>HHHHHHLPEKTIRWCVVSDHEATKCSSFRDNMKKVLPAGGPAVTCVRKMSHPECIRDISANKVDAVTVDGALVAEADLPHHSLKPIMAEYYGSKDDPKTHYYVVAMAKKGTGFQLNQLRGKKSCHTGLGWSAGWYVPLSTLLPSGSRETAAATFFSSSCVPCADGKMFPSLCQLCAGKGTDKCACSSREPYFGSWGALKCLQDGTADVSFVKHLTVFEAMPTKADRDQYELLCMDNTRRPVEEYEQCYLARVPSHVVVARSVDGKEDSIQELLRVAQEHFGKDKSSPFQLFGSPHGEDLLFTDAAHGLLRVPRKIDISLYLGYEFLSAFRNLKRGLEDSQRVKWCAVGQQERTKCDQWSAVSGGALACATEETPEDCIAATMKGEADAMSLDGGFAYVAGHCGLVPVLAENYLSTHSSGRLGSKCVNAPLEGYYVVAVVKKSDVGITWKSLQGKKSCHTAVGTSEGWNVPMGLIYDQTGSCKFDAFFSRSCAPGSDPDSPLCALCVGGNNPAHMCAANNAEGYHGSSGALRCLVEKGDVAFMKHPTVLQNTDGKNPEPWAKGLKHEDFELLCLDGTRKPVTEAQSCHLARVPNRAVFSRKDKADFVRRILFNQQELFGRNGFEYMMFQMFESSAKDLLFSDDTECLSNLQDKTTYKTYLGPQYLTLMDN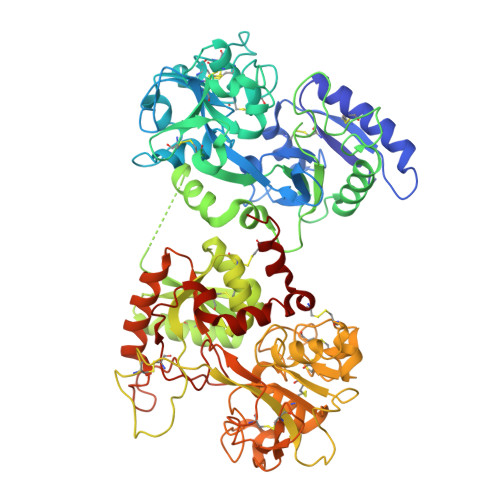FRQCLSSELLDACTFHKY[4x]> MGKYDGSKLRIGILHARWNAEIILALVLGALKRLQEFGVKRENIIIETVPGSFELPYGSKLFVEKQKRLGKPLDAIIPIGVLIKGSTMHFEYICDSTTHQLMKLN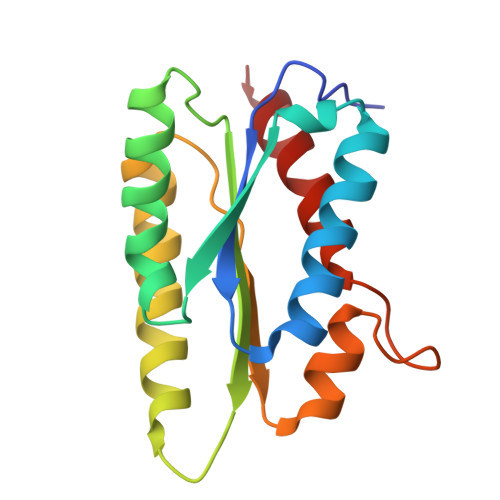FELGIPVIFGVLTCLTDEQAEARAGLIEGKMHNHGEDWGAAAVEMATKFN> GKLSLQDVAELIRARACQRVVVMVGAGISTPSGIPDFRS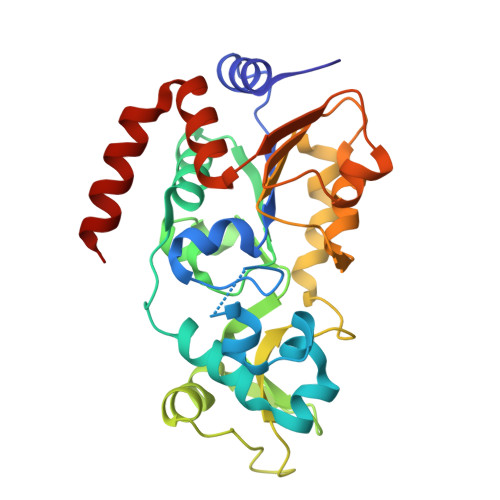PGSGLYSNLQQYDLPYPEAIFELPFFFHNPKPFFTLAKELYPGNYKPNVTHYFLRLLHDKGLLLRLYTQNIDGLERVSGIPASKLVEAHGTFASATCTVCQRPFPGEDIRADVMADRVPRCPVCTGVVKPDIVFFGEPLPQRFLLHVVDFPMADLLLILGTSLEVEPFASLTEAVRSSVPRLLINRDLVGPLAWHPRSRDVAQLGDVVHGVESLVELLGWTEEMRDLVQRETGKLA> TRSGKVM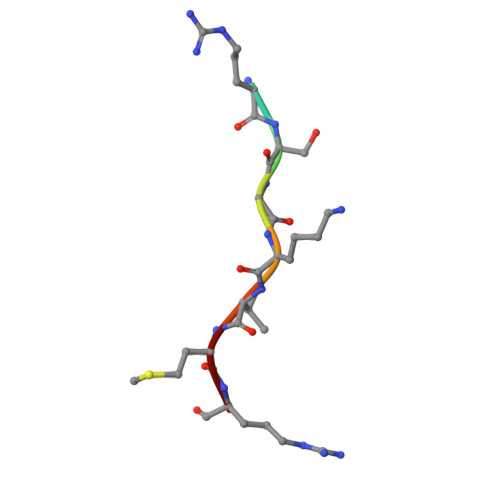R>SDKQKAINYLMQFAHKVSGKYRGVAKLEGNTKAKVLQVLATFAYADYCRSAAT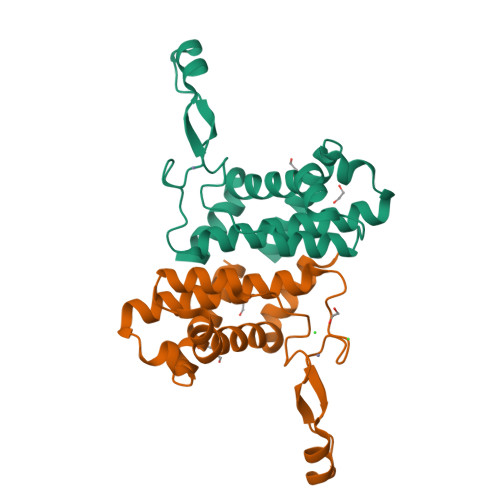PGARCRDCHGTGRAVDIAKTKLWGRVVEKECGRCKGVGYSRMPASAAYRAVTMLIPNLTQPTWSRTVKPLYDALVVQCHKEESIADNILNAVTR[2x]The protein N is a multifunctional protein that packs the genomic RNA and enhances the efficiency of virus transcription and assembly. N contains an N-terminal domain, involved in RNA binding, and a C-terminal (NCTD) involved in RNA binding, protein dimerization, and interaction with the viral membrane protein (M). The SARS-CoV-2 NCTD folds into a helical core with a protruding β-hairpin employed for protein dimerization. Here we report the crystal structure of the C-terminal domain (NCTD) in open and closed conformations and in complex with guanine triphosphate, GTP.

The crystal structure of NCTD was solved by molecular replacement to a resolution of 1.94 Å. The crystal asymmetric unit contains two homodimers of NCTD with almost identical conformation (rmsd 0.14 Å). Two monomers are intertwined through the β-hairpin forming a four antiparallel β-sheet on one face of the dimer. In striking contrast to the previously described structures, the superposition of the subunits in our structure shows a ≈5.5 Å movement of the β-hairpin. One subunit presents the β-hairpin in an extended and previously unseen conformation that we named “open”. Whereas the other subunit shows a β-hairpin in a flexed conformation that we named “closed”, similar to other structures of this protein. The alternative conformation of the β-hairpin is associated with the structural displacement of the loop between α1 and α2 (residues 280–283). In the closed conformation the β-hairpin interacts with the C-terminal proline residue (P364) of a symmetry-related protein. This interdimeric interaction between W330 and P364 through a π–π stacking (face-to-face rings interaction), and making hydrogen bonds with T325 and S327, is a common feature with seven NCTD structures determined previously. But strikingly, our structure shows that in the open conformation, the side chain of the residue W330 is rotated 180° towards the β-hairpin making hydrophobic contacts with the side chain of the residues T325 and S327. Therefore, our structure shows that upon a side-chain arrangement the β-hairpin changes from an open conformation to a closed conformation that might favor the interdimeric interaction.

>MGSSHHHHHHGENLYFQSTKKSAAEASKKPRQKRTATKAYNVTQAFGRRGPEQTQGNFGDQELIRQGTDYKHWPQIAQFAPSASAFFGMSRIGMEVTPSGTWLTYTGAIKLDDKDPNFKDQVILLNKHIDAYKTFP[4x]>SNAMIRKYRYGAPFDTEALTEKIETAEEAFPYGEISQKEGFAFTYIMDEDDIVYGLGESNRGINKRGYCYISNCTADPIHTEDKRSLYGAHNFIIVSGKTTFGLFFDYPSKLTFDIGYTRMDTLKVSCENADLDIYVIEGENAYDIVKQFRRVIGRSYIPPKFAFGFGQSRWGYTTKEDFRAVAKGYRENHIPIDMIYMDIDYMQDFKDFTVNEKNFPDFPEFVKEMKDQELRLIPIIDAGVKVEKGYEVYEEGVKNNYFCKREDGSDFVAAVWPGDTHFPDMLNPEARKWFGDKYRFLIDQGIEGFWNDMNEPAIFYSSEGLAEAKEFAGEFAKDTEGKIHPWAMQAKMKDIVNSPEDYKRFYHNVNGKKIRHDKVHNLFGYNMTRAAGEAFERIDPEKR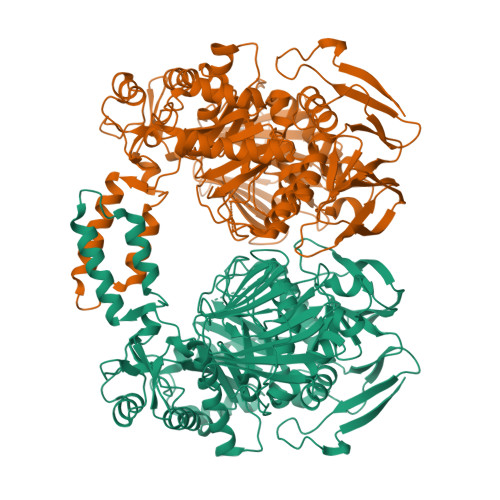FLMFSRSSYIGMHRYGGIWMGDNKSWWSHILLNLKMLPSLNMCGFMYTGADLGGFGDDTTRDLLLRFLALGVFTPLMRDHAAEGTREQECYQFENIEDFRSVINARYRLVPYLYSEYMKAALNDDMYFKPLGFVYPDDKMAIRVEDQLMLGNEIMIAPVYEQNARGRYVYLPEEMKFIKFMPDGSISEEVLEKGVHYVDVALNEVPLFIRSGKCIPVAEAAECVKDIDTENMQLIGYEGSSYTLYEDDGIHKDYDKKENYRVLTK[2x]> HHHHHHMAEVKLYGFWPSPFSHRIIWALKLKGVEYEYIEEDLSNKSESLLKYNPVYKKTPVLVHGDKPIAESLVILEYIEETWPENPLLPKDPYERAMARFWIQYGVDTVAALRAFYLGSG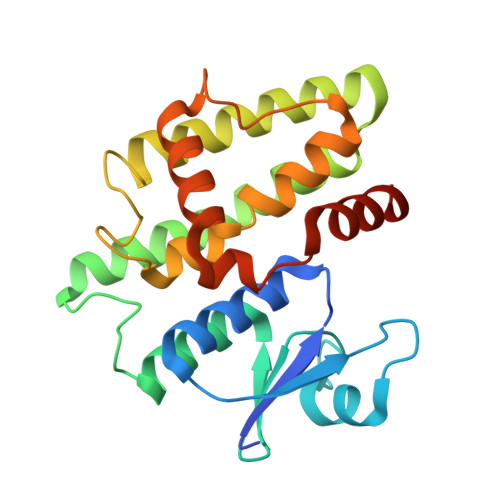EELEKAAKELSECLKILEEQGLGDKKFFGGESMNLVDISYGALGYWLAAVEEAKGVTVLKPSTLPRLHAWAKNLDELPVVKENIPASDKMLAYVTAAMNRPAKN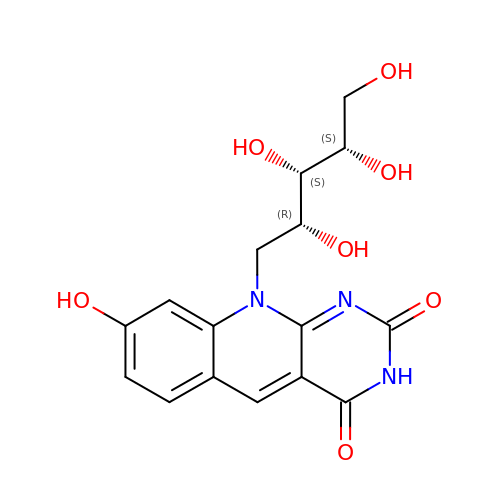8-HYDROXY-10-(D-RIBO-2,3,4,5-TETRAHYDROXYPENTYL)-5-DEAZAISOALLOXAZINE | C16 H17 N3 O7 | AUEILLWDYUBWCM-AGIUHOORSA-N>[3x]MKMVVAVIRPEKLECVKKALEERGFVGMTVTEVKGRGEQKGIRLQFRGREVEVDLLQ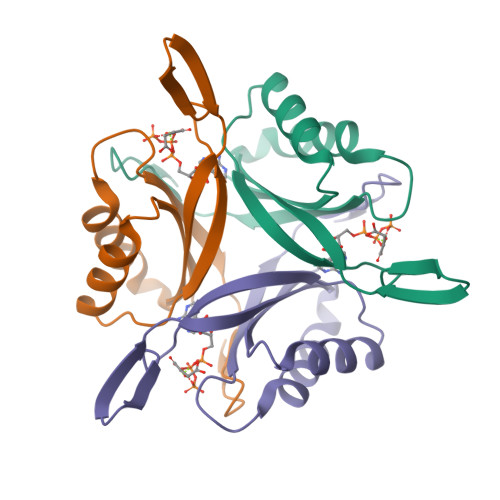KTKVEVVVSDDAVDEVVEAIVSSARTGKFGDGRIFVIPVEKSVKIRTGDEEVAAAHHHHHH> SMVLLTMIARVADGLPLAASMQEDEQSGRDLQQYQSQAKQLFRK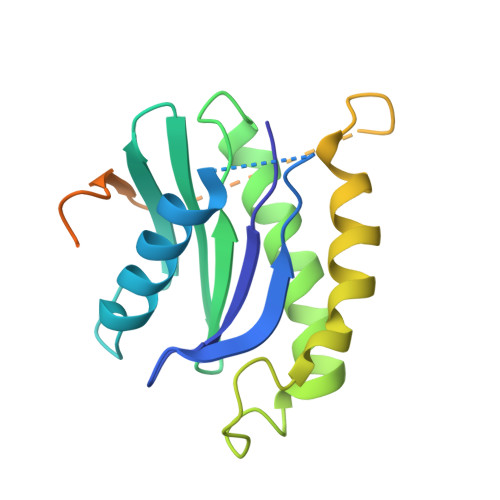LNEQSPTRCTLEAGAMTFHYIIEQGVCYLVLCEAAFPKKLAFAYLEDLHSEFDEQHGKKVPTVSRPYSFIEFDTFIQKTKKLYIDSRARRNLGSINTELQDVQRIMVANIEEVLQRGEALSALDSKANNLSSLSKKYRQDAKYLNMRSTYAK>[2x]MGSSHHHHHHHSSGLVPRGSHHMLEMQINLPEVHAEVTAQFVRYEKALTSNDTAVLNELF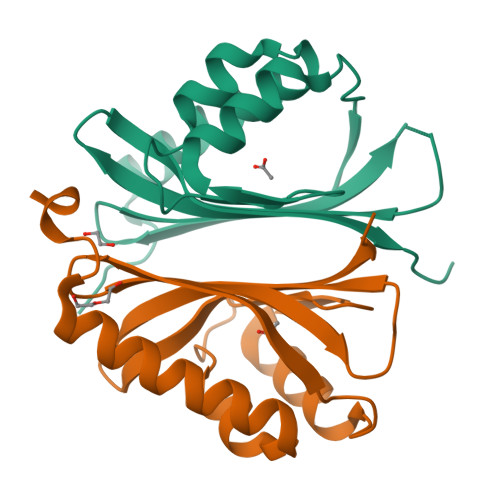WNSPQTLRYGATENLYGYEAIAGFRATRSPNNLEREIVRTVITTYGHDFATANIEFRRLSHSQLTGRQSQTWMRTSQGWRVVAAHVSLIALPVS>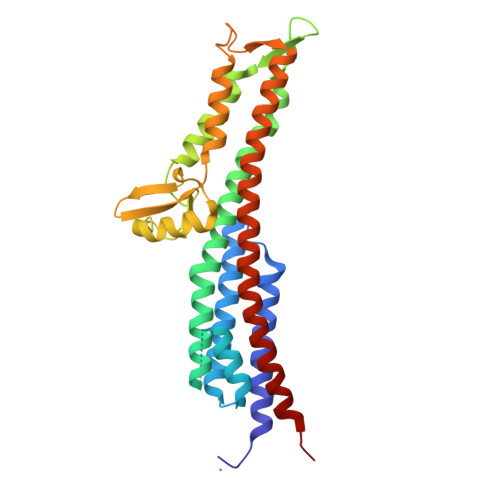[2x]GHMEHRGTDIISLSQAATKIHQAQQTLQSTPPISEENNDERTLARQQLTSSLNALAKSGVSLSAEQNENLRSAFSAPTSALFSASPMAQPRTTISDAEIWDMVSQNISAIGDSYLGVYENVVAVYTDFYQAFSDILSKMGGWLLPGKDGNTVKLDVTSLKNDLNSLVNKYNQINSNTVLFPAQSGSGVKVATEAEARQWLSELNLPNSCLKSYGSGYVVTVDLTPLQKMVQDIDGLGAPGKDSKLEMDNAKYQAWQSGFKAQEENMKTTLQTLTQKYSNANSLYDNLVKVLSSTISSSLETAKSFLQG> MTDISQMYDQLSDPFAGLGAGNIHLGYFDGPDDAATLAEAADRLTDQLIARLPVVRDHRVLDVGCGVGKPALRLAGDLGVRVVGVSISEAQIGIANEAARAAGLADRVSFRYADAMRLPFPDASFDGVWAMESLHHMPDRLQALREIARVLRHGGVLSIAD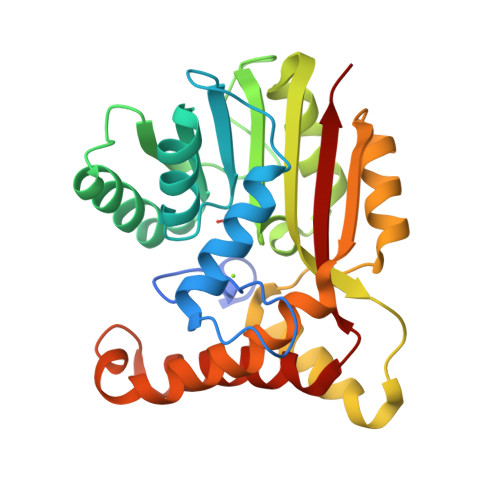FVQLGPVREQDEEALRAFRSGGGVHTLTGIAEYEAEIADAGLTLTSSSDISANVRPSMVRTAEAIRGAADAFLPLMGEEGLRRLIDNFERAATVPQIGYALFAARRS>GPTIYHAKDAVQATKPDMRKPRLVVFVVGETARADHVSFNGYERDTFPQLAKIDGVTNFSNVTSCGTSTAYSVPCMFSYLGADEYDVDTAKYQENVLDTLDRLGVSILWRDNNSDSKGVMDKLPKAQFADYKSATNNAICNTNPYNECRDVGMLVGLDDFVAANNGKDMLIMLHQMGNHGPAYFKRYDEKFAKFTPVCEGNELAKCEHQSLINAYDNALLATDDFIAQSIQWLQTHSNAYDVSMLYVSDHGESLGENGVYLHGM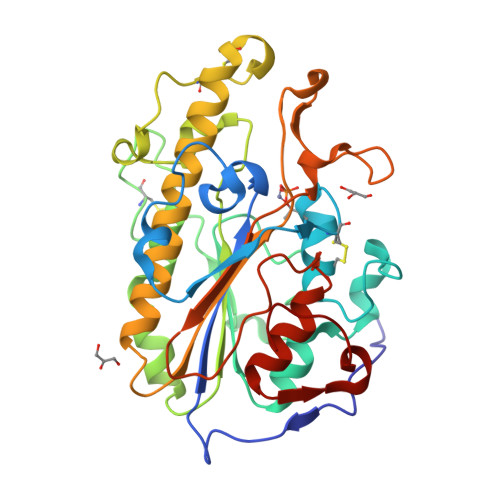PNAFAPKEQRSVPAFFWTDKQTGITPMATDTVLTHDAITPTLLKLFDVTADKVKDRTAFIR[2x]> AKEEIIWESLSVDVGSQGNPGIVEYKGVDTKTG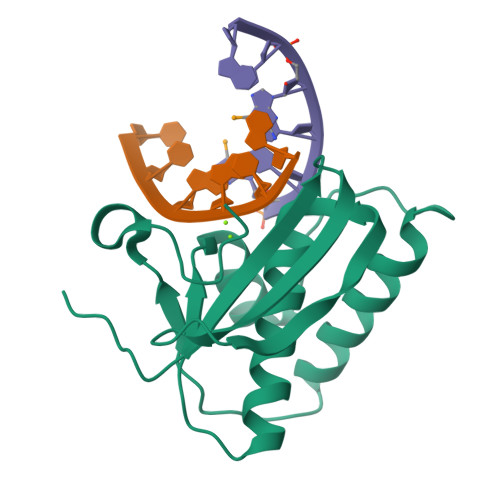EVLFEREPIPIGTNNMGEFLAIVHGLRYLKERNSRKPIYSNSQTAIKWVKDKKAKSTLVRNEETALIWKLVDEAEEWLNTHTYETPILKWQTDKWGEIKADYGRK> MVGLTTLFWLGAIGMLVGTLAFAWAGRDAGSGERRYYVTLVGISGIAAVAYVVMALGVGWVPVAERTVFAPRYINWILTTPLIVYFLGLLAGLDSREFGIVI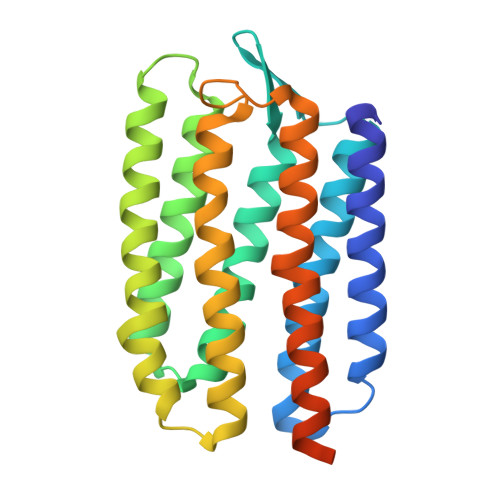TLNTVVMLAGFAGAMVPGIERYALFGMGAVAFLGLVYYLVGPMTESASQRSSGIKSLYVRLRNLTVILWAIYPFIWLLGPPGVALLTPTVDVALIVYLDLVTKVGFGFIALDAAATLRAEHGESLAGVDTDAPAVADHHHHHH>XNRVFAEYPDHIQDYFKQSFPKGYSWERSLTFEDGGICIARNDITMEGDTFYNKVRFHGVNFPANGPVMQKKTLKWEPSTEKMYVRDGVLTGDITMALLLEGNAHYRCDSRTTYKAKEKGVKLPGYHLVDHCIEILSHDKDYNKVKLYEHAVAHSGLPDNARR[4x];>HHMSAIKPDMKINLRMEGNVNGHHFVIDGDGTGKPFEGKQSMDLEVKEGGPLPFAFDILT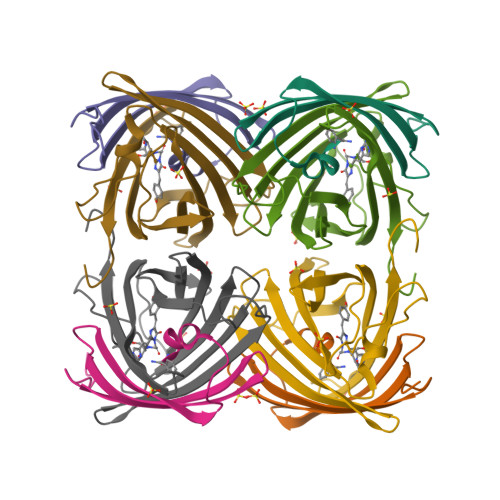TAF[4x]> SMETNPIPVVTVQTTPFDDQKPGTNGLRKKTTVFESK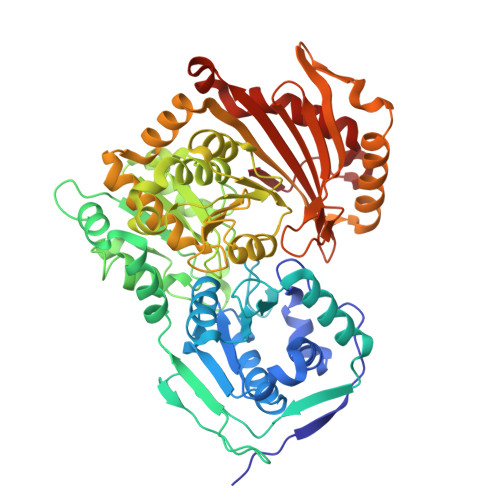KNYLQNYIQSVLSSIDLRDRQGCTMVVGSDGRYFSRTAIEVIVQMAAANGIGRLVIGHNGILSTPAVSCIIRKIKAIGGIILTASRNPGGPNGDFGIKFNVANGGPAPDTVIDKIHQVSRTLEEYAICPDMRIDLSRLGRQDFDLENKFKPFRVEIVDSVEVYLNLLRGIFDFNAIKGLLTGPDQLKMRVDAMSGVMGPYVRRILCDELGAPANSAVNCVPLEDFGGHYPDPNLTYATGLVDAMKGGEFGFGAAFDADGDRCMILGQNAFFVNPSDSLAVVAANLSCIPYFRQAGVRGFARSMPTSTAIDRVAKAMKVAVYETPAGWRFFGNLMDSGRCSFCGEESFGMGSDHIREKDGLWTVLVWLSIMAARKQGVEDIVRDHWTKLGRNYFCRFDYEAIDPRAAFYLMKDLEAVISDKAFCSQKFAVGNSVYSVEKADNFEYIDPVDGTVARNQGLRIIFSESSRLIFRLSGTGVGVGATIRIYAESFERDPERHNREPQVVLGPLIAIALKISDIHERTGRRGPTVIT> GGVVLRVVTVLEEPFVMVSENVLGKPKKYQGFSIDVLDALSNYLGFNYEIYVAPDHKYGSPQEDGTWNGLVGELVFKRADIGISALTITPDRENVVDFTTRYMDYSVGVLLRRGTSIQSLQDLSKQTDIPYGTVLDSAVYQHVRMKGLNPFERDSMYSQMWRMINRSNGSENNVLESQAGIQKVKYGNYAFVWDAAVLEYVAINDPDCS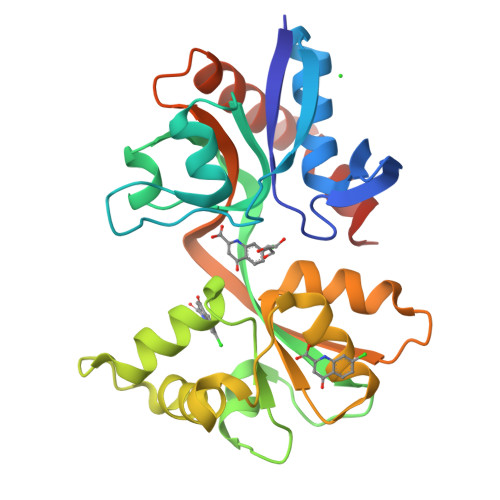FYTVGNTVADRGYGIALQHGSPYRDVFSQRILELQQSGDMDILKHKWWPKNGQCDL>[2x]MSEPVVVVGAGPAGLMLACELAMRDVPAVLVDIHPTQRAEAPAMAINAGTLEMLDQRGLAAGLREGTVTFPEVRFADLRLAFEKVQGPREPTHMVLQSRLEKVLIDRAVELGVDLRWATRLTGFEEAADGSGVTVTLASDAGEEQLRCRYLVGCDGRESIVRKQAGIDYVGDDWVIVRGIVGDVAINREDVAPEQYGLSYTDNGDQFLG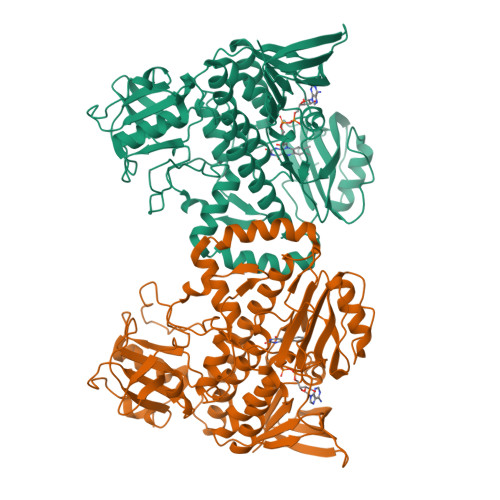APLSPDVMRVFSAEFSTEPPEFEDGPATLEQLGDAVKRLTGKELKATEAHWLQHYSIVTRNAEQYRKGRVFIAGDAAHVHYPYNGQGLGTAIGDAVNLGWKIAAEVHGWAPADLLDSYHVERHLAGRLACMNIQAQLALLYPRPLARYMREMMGEFLKFDEVNVFLAEIVTNLGPAVPIAYEGVPEPVEGDRLLGRRLPKVQIKTADGDMGVAETLQSGRGVLLDLSGDASAQEESGWADRVDVVRAQPVPDLPGTLLLRPDGCVAWHDGGGWGQDELRTALRTWFGAPTG>TTTVGLVCKDGVVMATEKRATMGNFIASKAAKKIYQIADRMAMTTAGSVGDAQFLARIIKIEANLYEIRRERKPTVRAIATLTSNLLNSYRYFPYLVQLLIGGIDSEGKSIYSIDPIGGAIEEKDIVATGSGSLTAYGVLEDRFTPEIGVDEAVELAVRAIYSAMKRDSASGDGIDVVKITEDEFYQYSPEEVEQILAKFRK[14x];>QMGYDRAITVFSPDGRLFQVEYAREAVKRGATAIGIKCKEGVILIADKRVGSKLLEADTIEKIYKIDEHICAATSGLVADARVLIDRARIEAQINRLTYDEPITVKELAKKICDFKQQYTQYGGVRPFGVSLLIAGVDEVPKLYETDPSGALLEYKATAIGMGRNAVTEFFEKEYRDDLSFDDAMVLGLVAMGLSIESELVPENIEVGYVKVDDRTFKEVSPEELKPYVERANERIRELLKK[14x];>LLEKLKKLEEDYYKLRELYRRLEDEKKFIESERIRYEREVRRLRSEVERLRSPPLLVGVVSDILEDGRVVVKSSTGPKFVVNTSQYI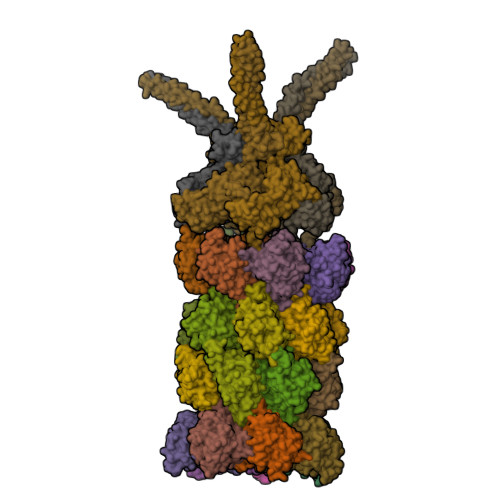NEEELKPGARVALNQQTLAIVNVLPTSKDPMVYGFEVEEKPEVSYEDIGGLDVQIEEIREAVELPLLKPELFAEVGIEPPKGVLLYGPPGTGKTLLAKAVANQTRATFIRVVGSEFVQKYIGEGARLVREVFQLAKEKAPSIIFIDELDAIAARRTNSDTSGDREVQRTMMQLLAELDGFDPRGDVKVIGATNRIDILDPAILRPGRFDRIIEVPLPTFEGRIQIFKIHTRKMKLAEDVDFKELARITEGASGADIKAICTEAGMFAIREERAKVTMLDFTKAIEKVLKKTTPIPDLKGVMFV[6x]>[2x]MMEGVKDFKQELLLV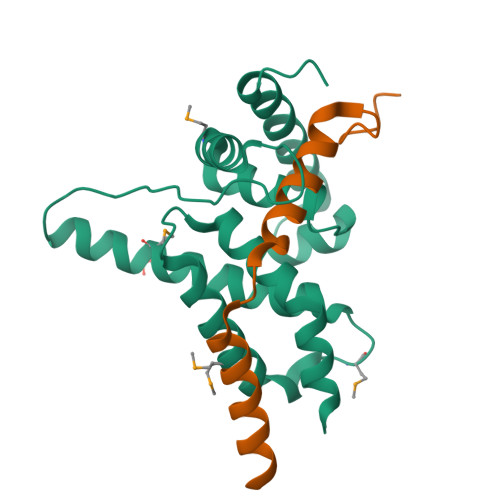LPALRAFAISLSSKHDKAEDLVQDTLMKAWAKQDSFEMGSNLKAWLFTILRNEFYSQMRKRGREVQDSDGVFIESVAIHPAQYGSLDLQDFKKALNMLSADQREAIILIGASGFSYEDAAAICGCAIGTIKSRVSRARNRLQELLKVDR;>MNDCDEKNLTNHFTFGDDLLGVNSEIARKLRQFYLEIQEEALPARLLELLERLEQAERFGLNNAEKV[2x]> GHHHHHHMIEWIIRRSVANRFLVLMGALFLSIWGTWTIINTPVDALPDLSDVQVIIKTSYPGQAPQIVENQVTYPLTTTMLSVPGAKTVRGFSQFGDSYVYVIFEDGTDPYWARSRVLEYLNQVQGKLPAGVSAELGPDATGVGWIYEYALVDRSGKHDLADLRSLQDWFLKYELKTIPDVAEVASVGGVVKEYQVVIDPQRLAQYGISLAEVKSALDASNQEAGGSSIELAEAEYMVRASGYLQTLDDFNHIVLKASENGVPVYLRDVAKVQIGPEMRRGIAELNGEGEVAGGVVILRSGKNAREVIAAVKDKLETLKSSLPEGVEIVTTYDRSQLIDRAIDNLSGKLLEEFIVVAVVCALFLWHVRSALVAIISLPLGLCIAFIVMHFQGLNANIMSLGGIAIAVGAMVDAAIVMIENAHKRLEEWQHQHPDATLDNKTRWQVITDASVEVGPALFISLLIITLSFIPIFTLEGQEGRLFGPLAFTKTYAMAGAALLAIVVIPILMGYWIRGKIPPESSNPLNRFLIRVYHPLLLKVLHWPKTTLLVAALSVLTVLWPLNKVGGEFLPQINEGDLLYMPSTLPGISAAEAASMLQKTDKLIMSVPEVARVFGKTGKAETATDSAPLEMVETTIQLKPQEQWRPGMTMDKIIEELDNTVRLPGLANLWVPPIRNRIDMLSTGIKSPIGIKVSGTVLADIDAMAEQIEEVARTVPGVASALAERLEGGRYINVEINREKAARYGMTVADVQLFVTSAVGGAMVGETVEGIARYPINLRYPQSWRDSPQALRQLPILTPMKQQITLADVADIKVSTGPSMLKTENARPTSWIYIDA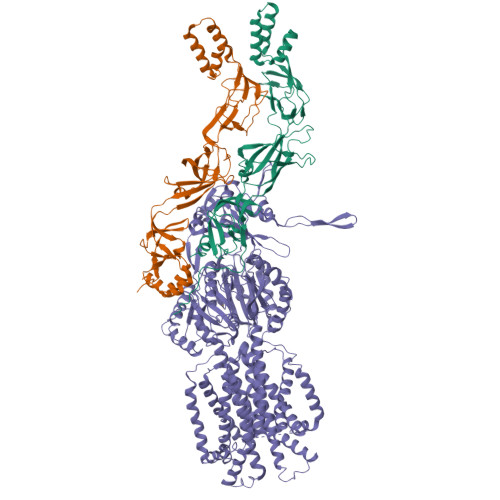RDRDMVSVVHDLQKAIAEKVQLKPGTSVAFSGQFELLERANHKLKLMVPMTLMIIFVLLYLAFRRVGEALLIISSVPFALVGGIWLLWWMGFHLSVATGTGFIALAGVAAEFGVVMLMYLRHAIEAVPSLNNPQTFSEQKLDEALYHGAVLRVRPKAMTVAVIIAGLLPILWGTGAGSEVMSRIAAPMIGGMITAPLLSLFIIPAAYKLMWLHRHRVRK;>[2x]SASGVRIDPTQTQNLGVKTATVTRGPLTFAQSFPANVSYNEYQYAIVQARAAGFIDKVYPLTVGDKVQKGTPLLDLTIPDWVEAQSEYLLLRETGGTATQTEGILERLRLAGMPEADIRRLIATQKIQTRFTLKAPIDGVITAFDLRAGMNIAKDNVVAKIQGMDPVWVTAAIPESIAWLVKDASQFTLTVPARPDKTLTIRKWTLLPGVDAATRTLQLRLEVDNADEALKPGMNAWLQLNTASEPMLLIPSQALIDTGSEQRVITVDADGRFVPKRVAVFQASQGVTALRSGLAEGEKVVSSGLFLIDSEANISGALERMRSESATHAHHHHHHH>[2x]MQGCPFAKRDGTVDSSLPQKRADAPETTTFGRCAVKSNQAGGGTRSHDWWPCQLRLDVLRQFQPSQNPLGGDFDYAEAFQSLDYEAVKKDIAALMTESQDWWPADFGNYGGLFVRMAXHSAGTYRAMDGRGGGGMGQQRFAPLNSWPDNQNLDKARRLIWPIKQKYGNKISWADLMLLTGNVALENMGFKTLGFGGGRADTWQSDEAVYWGAETTFVPQGNDVRYNNSVDINARADKLEKPLAATHMGLIYVNPEGPNGTPDPAASAKDIREAFGRMGMNDTETVALIAGGHAFGKTHGAVKGSNIGPAPEAADLGMQGLGWHNSVGDGNGPNQMTS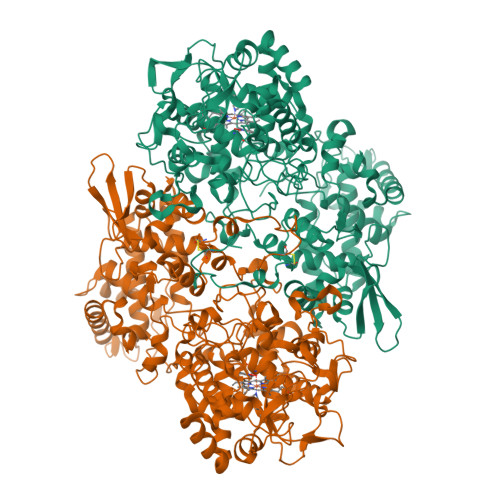GLEVIWTKTPTKWSNGYLESLINNNWTLVESPAGAHQWEAVNGTVDYPDPFDKTKFRKATMLTSDLALINDPEYLKISQRWLEHPEELADAFAKAWFKLLHRDLGPTTRYLGPEVPKESFIWQDPLPAREGDLIDDADVDKLKAAILSTDGLDVSKLASTAMACATTYRNSDKRGGCNGARIALEPQRNWVSNNPTQLSAVLDALKKVQSDFNGSNGNKKVSLADLIVLGGTAAVEKAAKDAGVDIKVPFSAGRVDATQEQTDVTQFSYLEPQADGFRNYGRGTARARTEEIMVDKASQLTLTPPELTVLVGGMRALGANYDGSDVGVFTANKGKLTPDFFVNLVDMNIAWTASGADGESWVGTDRKSRSEKYKGSRADLVFGSHAELRAIAEVYAENGNQEKFVKDFVAAWTKVMNLDRFDLKVKK>[2x]DERDRVQKKTFTKWVNKHLIKAQRHISDLYEDLRDGHNLISLLEVLSGDSLPREKGRMRFHKLQNVQIALDYLRHRQVKLV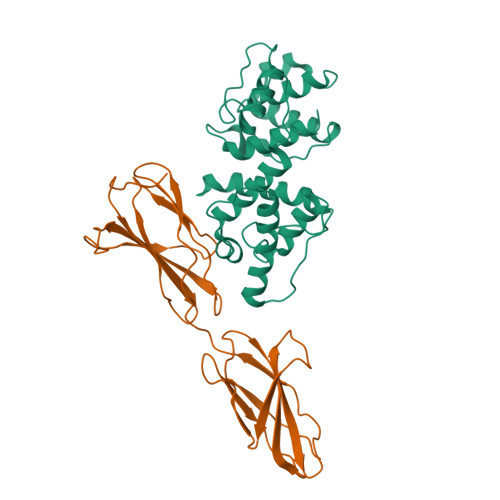NIRNDDIADGNPKLTLGLIWTIILHFQISDIQVSGQSEDMTAKEKLLLWSQRMVEGYQGLRCDNFTSSWRDGRLFNAIIHRHKPLLIDMNKVYRQTNLENLDQAFSVAERDLGVTRLLDPEDVDVPQPDEKSIITYVSSLYDAMP;>[2x]DLGAPQNPNAKAAGSRKIHFNWLPPSGKPMGYRVKYWIQGDSESEAHLLDSKVPSVELTNLYPYCDYEMKVCAYGAQGEGPYSSLVSCRTHQEVPSEPGRLAFNVVSSTVTQLSWAEPAETNGEITAYEVCYGLVNDDNRPIGPMKKVLVDNPKNRMLLIENLRESQPYRYTVKARNGAGWGPEREAIINLATQP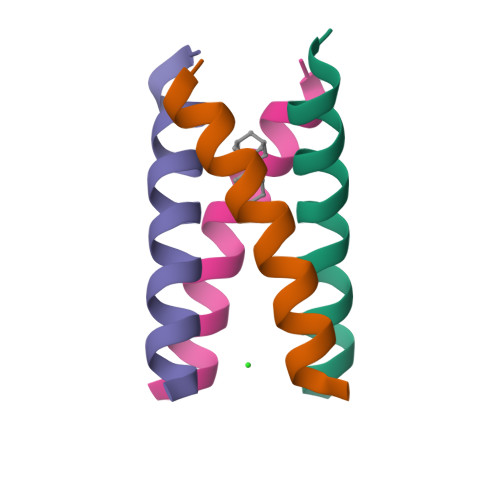>[16x]XSSDPLVVAASIIGILHLILWILDRLX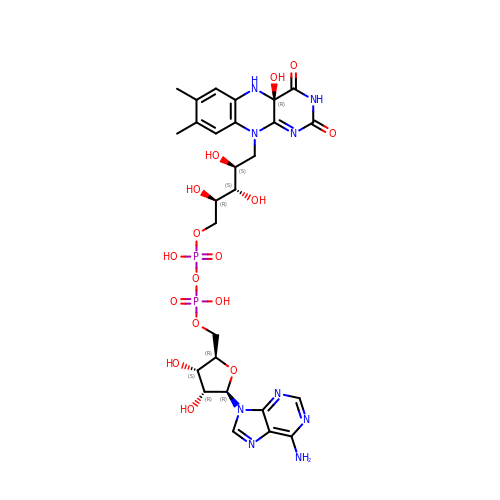[(2R,3S,4R,5R)-5-(6-amino-9H-purin-9-yl)-3,4-dihydroxytetrahydrofuran-2-yl]methyl (2R,3S,4S)-2,3,4-trihydroxy-5-[(4aR)-4a-hydroxy-7,8-dimethyl-2,4-dioxo-3,4,4a,5-tetrahydrobenzo[g]pteridin-10(2H)-yl]pentyl dihydrogen diphosphate (non-preferred name) | C27 H35 N9 O16 P2 | WTOYVZYXGAOYIM-QUWWARRSSA-N> MLIKKALTAVALLASLLGASAAFAFAHLKSATPAADSTVAAPADLRLTFSEGVEATFTKV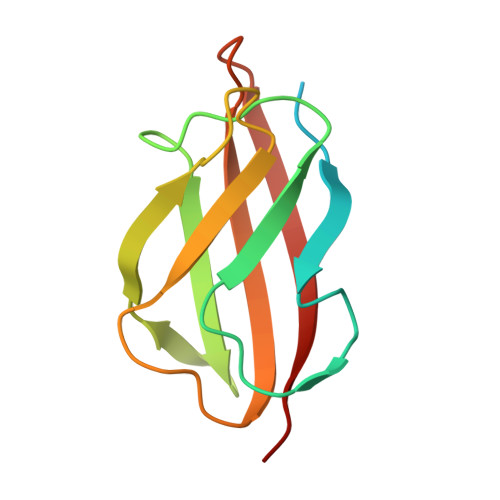SLSKDGTEVAIKGLETPDADKKTLVVTPAAPLAAGNYKVVWNAVSVDTFKSNGEYSFKVKKK>GPGSADPKPMVMWKDLLTGSWKGPDVLITAGRGYACVFPQDAESPIW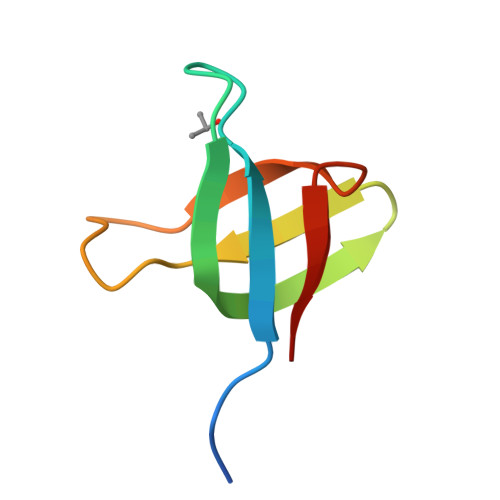VPDRFIRPFTE[2x]> AHKNRIFVSSSKDFEGYPSKAIVPVQFVALLTSIHLTETKCLLGFSNFERRGDQSQEDQYLIKLKFKDRGSERLARITISLLCQYFDIELPDLDSDSGASPTVILRDIHLERLCFSSCKALYVSKHGNYTLFLEDIKPLDLVSVISTISTKSTNSSKHSSSELISECDLNNSLVDIFNNLIEMNRDEKNRFKFVKLIHYDIELKKFVQDQQKVLSQKSKAAAINPFFVPN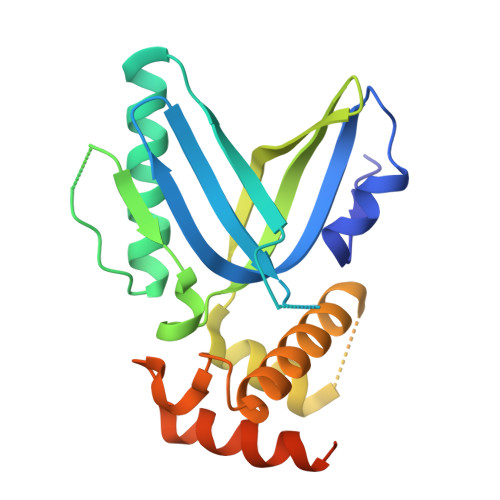RLG>[2x]MGADDVVDSSKSFVMENFSSYHGTKPGYVDSIQKGIQKPKSGTQGNYDDDWEGFYSTDNKYDAAGYSVDNENPLSGKAGGVVKVTYPGLTKVLALKVDNAETIKKELGLSLTEPLMEQVGTEEFIKRFGDGASRVVLSLPFAEGSSSVKYINNWEQAKALSVELEINFETRGKRGQDAMYEYMAQACAGNRVRRSVGSSLSCINLDWDVIRDKTKTKIESLKEQGPIKNKMSESPNKTVSEEKAKQYLEEFHQTALEQPELSELKTVTGTNPVFAGANYAAWAVNVAQVIDSETADNLEKTTAALSILPGIGSVMGIADGAVHHNTEEIVAQSIALSSLMVAQAIPLVGELVDIGFAAYNFVESIINLFQVVHNSYNRPAYSPGHKTQPFLHDGYAVSWNTVEDSIIRTGFQGESGHDIKITAENTPLPIAGVLLPTIPGKLDVNKSKTHISVNGRKIRMRCRAIDGDVTFCRPKSPVYVGNGVHANLHVAFHRSSSEKIHSNEISSDSIGVLGYQKTVDHTKVNSKLSLFFEIKSMA

Protonation of key histidine residues has been long implicated in the acid-mediated cellular action of the diphtheria toxin translocation (T-) domain, responsible for the delivery of the catalytic domain into the cell. The function of the T-domain is to translocate the catalytic domain across the lipid bilayer in response to the acidification of the endosome. Remarkably, such a complex task is performed by this small 180-residue protein without the help of any additional translocation machinery. Formation of the membrane-competent W+-state occurs in solution upon acidification of the environment to pH below 6 and is accompanied by structural destabilization and partial unfolding of the T-domain.

In order to further analyze the putative pH-dependent structuring of the TH2-TH3 region, we crystallized a full-length form of diphtheria toxin (DT) harboring the H223Q/H257Q mutations. Notably, two crystal forms were obtained from crystallization solutions at pH 5.5 and 4.5. The first crystal form (DT-DM-A) was isomorphous with the aforementioned WT structures, whereas the other form (DT-DM-B) belonged to another crystal form. Not surprisingly, the mutant structures also form domain-swapped dimers and are similar to the WT structures. Interestingly, the TH2 helices in the mutant structures are well ordered in a similar manner as observed for the WT pH 7.0 structure and could be modeled on the electron density maps. Interestingly, the Q223/Q257 sidechain conformations are distinctly different from the H223/H257 residues in the WT structures. Concerted movement of Q223, Q257, and E259 in DT-DM-B results in the formation of new hydrogen bond interactions, as shown in Figure 4. Moreover, the acid-induced destabilization of the T-domain’s short helix TH2, previously reported for the WT, is no longer observed with the DM. The latter is overall consistent with the spectroscopic evidence presented above in Figure 2 for the lack of efficient conversion of the membrane-competent state in the mutant.9-(3-azanylpropyl)-8-bromanyl-purin-6-amine | C8 H11 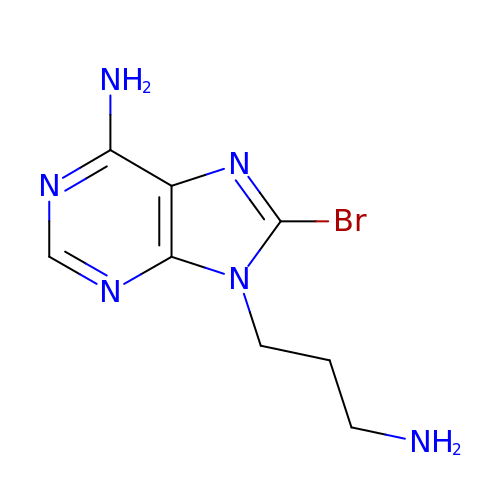Br N6 | PUSZSAUISWVTAT-UHFFFAOYSA-N> AYASDGSDQADLVSATEEAKDEKSEEPTPSETPTETETATPTTDHDCGKAGEYQKDLETTLASLADYG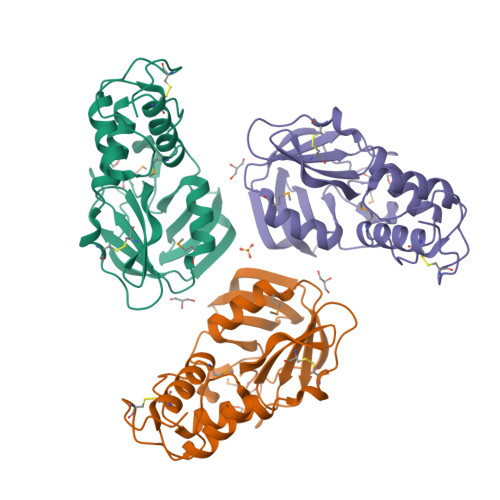TIFADGKQSKEDCAAIKKFQKRMGIQPAEGYAGKLTLDVAQRIAKSSFDKCQEAKKGKTVCVDLTHQTLWVVEDGKRIFEPTVVRTGMAGYATQPGAWKIFVKEGTHWSKKYKVWLPYWQNFNNGEGLHTTTTYIHEPWIGSHGCVNLLPSDSKKLYEMLDFGDTVQVFGNRPGT> AMEVHPISEFASPFEVFKCIERDFKVAGLLESIGGPQYKARYSVIAWSTNGYLKIHDDPVNILNGYLKDLKLADIPGLFKGGMIGYISYDAVRFWEKIRDLKPAAEDWPYAEFFTPDNIIIYDHNEGKVYVNADLSSVGGCGDIGEFKVSFYDESLNKNSYERIV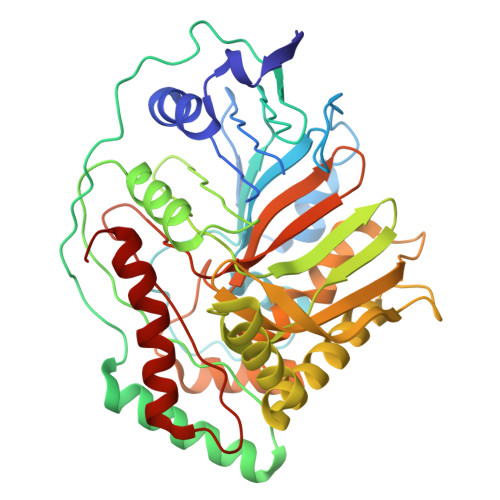SESLEYIRSGYIFQVVLSRFYRYIFSGDPLRIYYNLRRINPSPYMFYLKFDEKYLIGSSPELLFRVQDNIVETYPIAGTRPRGADQEEDLKLELELMNSEKDKAEHLMLVDLARNDLGKVCVPGTVKVPELMYVEKYSHVQHIVSKVIGTLKKKYNALNVLSATFPAGTVSGAPKPMAMNIIETLEEYKRGPYAGAVGFISADGNAEFAIAIRTAFLNKELLRIHAGAGIVYDSNPESEYFETEHKLKALKTAIGVR>[2x]IGTGFPFDPHYVEVLGERMHYVDVGPRDGTPVLFLHGNPTSSYVWRNIIPHVAP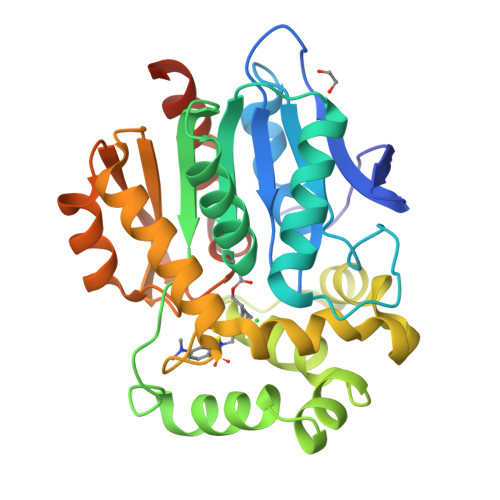THRCIAPDLIGMGKSDKPDLGYFFDDHVRFMDAFIEALGLEEVVLVIHDWGSALGFHWAKRNPERVKGIAFMEFIRPIPTWDEWPEFARETFQAFRTTDVGRKLIIDQNVFIEGTLPMGVVRPLTEVEMDHYREPFLNPVDREPLWRFPNELPIAGEPANIVALVEEYMDWLHQSPVPKLLFWGTPGVLIPPAEAARLAKSLPNCKAVDIGPGLNLLQEDNPDLIGSEIARWLSTLEISGLEISGLEHHHHHH>MKMLEQLEKKLGYTFKDKSLLEKALTHVSYSKKEHYETLEFLGDALVNFFIVDLLVQYSPNKREGFLSPLKAYLISEEFFNLLAQKLELHKFIRIKRGKINETIIGDVFEALWAAVYIDSGRDANFTRELFYKLFKEDIL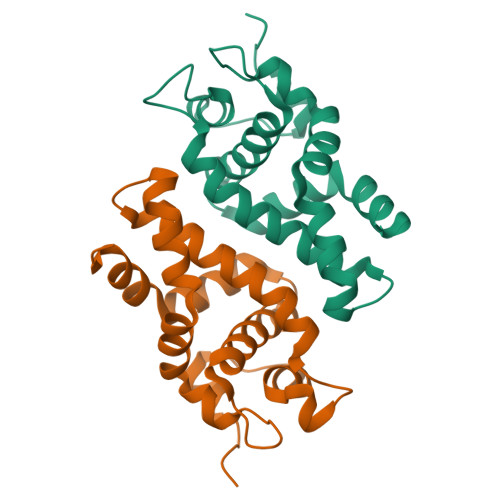SAIKEGR[2x]> ETGGSWAQVKLLESGGKVTHEGQSVTLTCKASGFNFKDYDMSWHWSPSGSNRQLVASISSKTGSKTEYKPRIQGRAYITRNNEANTVSLTLIQLRKEDSGIYYCAKLENVGGLSRYIIREQWGNFGPGTKLTVLPLEKTLLTESGGGT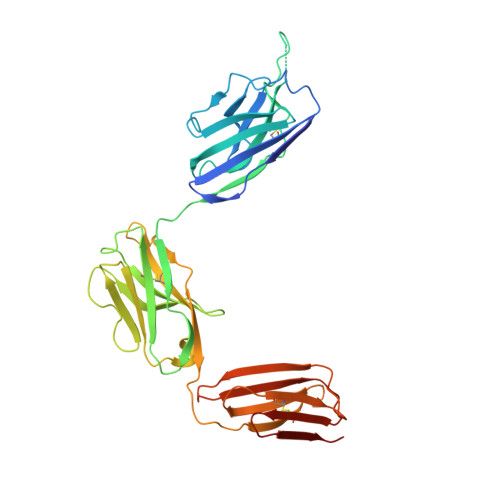YQAGKTLSLKCQTSGFQFKTSQLDWYLWTPGHAPLWLTGLNSSSTDATEGRITSSREDNKNQIFLQIEDLGLRDSGQYHCARRVGNGDDTDKLVFGLGTRVIVEPRPQAPLSPSVFLVRDQNAVACLIRNFYPKELHVSLTSSGTLISAQNLTLAPMATGTYSAIHIGRVGENDAITCSVKHLEKEIHMSHQAGSLVPR>[4x]GSHEATVEYLADLVKEKKHLTLFPHMFSNVERLLDD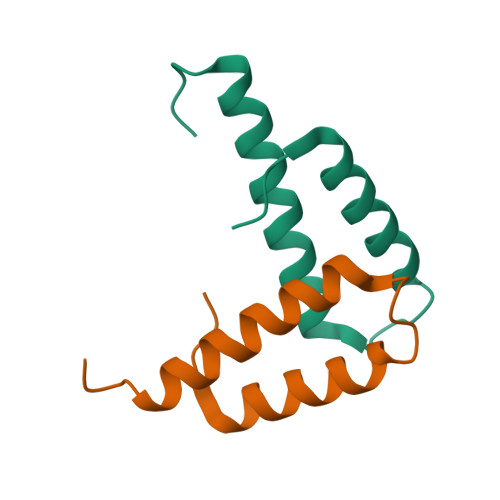EIGRVRVALFQTEFPRVELPEPAG>[2x]GSHMKLHERLRELRSERGLRLKDVAETAGISVPYLSDLERGRTNPSLETLQTLAGAYSITVHDLLEGVEFYGDSTEGALPKG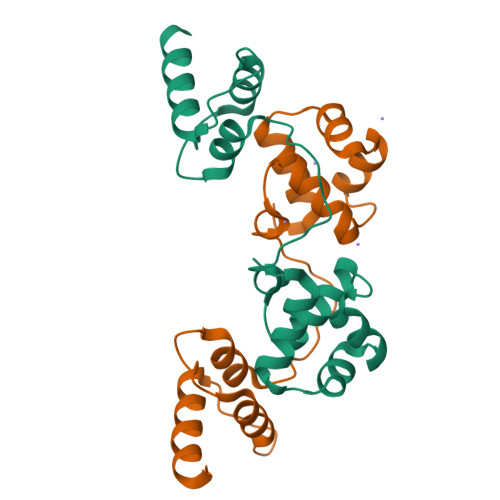LADLVADPLLGSQITPDWVRTLSRIELRGKRPRDKQDWYEIYLHLKRILG All bacteria contain a protein called YidC that inserts proteins into the plasma membrane of bacterial cells. At present, a mechanistic understanding of the function of YidC, as well as its mitochondrial and chloroplast counterparts Oxa1 and Alb3, respectively, is limited by a lack of structural information. Furthermore, the region(s) of YidC mediating the interaction with the ribosome have not been identified, and the oligomeric state of YidC during co-translational translocation remains controversial. In the resulting model, the conserved membrane integrated core of YidC forms a helical bundle arranged like the vertices of a pentagon, in the order 4-5-3-2-6 (clockwise) when viewed from the cytoplasm.

In order to provide a molecular model of YidC in its active state, we reconstituted purified full length YidC (extended with the C-terminus of R. baltica YidC [Seitl et al., 2014]) with ribosome nascent chains (RNCs) exposing the first TM helix of FOc, and subjected the complex to cryo-EM and single particle analysis to a resolution of ∼8 Å. In agreement with previous structural studies, YidC binds to the ribosomal exit site, however, the improved resolution now allows for a more detailed interpretation. Secondly, the presence of elongated structural features allowed us to dock our molecular model in a distinct orientation (cross correlation coefficient 0.865). Following placement of the YidC-core model, two prominent densities in the membrane region, one next to TM3 and one next to TM5, remained unaccounted for. Given that (i) YidC substrates are known to crosslink to TM3, and (ii) that the density neighboring TM3 is aligned with the ribosomal exit tunnel and (iii) that at the same relative position nascent chains have been observed inside the SecY channel, the most plausible assignment to the density near TM3 appeared to be the TM helix of FOc. To verify this, and to exclude that the density neighboring TM5 corresponds to the nascent chain, we reconstituted single cysteine mutants of YidC either in TM3 (M430C and P431C) or in TM5 (V500C and T503C) with RNCs of a single cysteine mutant of FOc(G23C), and exposed them to disulphide crosslinking. Thus, the adduct represented indeed the inserting FOc TM domain crosslinked to TM3 of YidC. Indeed, mutation of residues Y370A and Y377A (contacting ribosomal RNA helix 59) and D488K (contacting ribosomal protein uL23) severely interfere with YidC activity thereby emphasizing their functional significance. Finally, it is notable that we observe only a single monomer of YidC bound to the active ribosome. While SecY is known to translocate hydrophilic nascent chains through its central aqueous channel and insert TM domains through a lateral gate, our model suggests that the YidC substrates are inserted at the protein-lipid interface.

> MDSQRNLLVIALLFVSFMIWQAWEQDKNPQPQAQQTTQTTTTAAGSAADQGVPASGQGKLISVKTDVLDLTINTRGGDVEQALLPAYPKELNSTQPFQLLETSPQFIYQAQSGLTGRDGPDNPANGPRPLYNVEKDAYVLAEGQNELQVPMTYTDAAGNTFTKTFVLKRGDYAVNVNYNVQNAGEKPLEISSFGQLKQSITLPPHLDTGSSNFALHTFRGAAYSTPDEKYEKYKFDTIADNENLNISSKGGWVAMLQQYFATAWIPHNDGTNNFYTANLGNGIAAIGYKSQPVLVQPGQTGAMNSTLWVGPEIQDKMAAVAPHLDLTVDYGWLWFISQPLFKLLKWIHSFVGNWGFSIIIITFIVRGIMYPLTKAQYTSMAKMRMLQPKIQAMRERLGDDKQRISQEMMALYKAEKVNPLGGCFPLLIQMPIFLALYYMLMGSVELRQAPFALWIHDLSAQDPYYILPILMGVTMFFIQKMSPTTVTDPMQQKIMTFMPVIFTVFFLWFPSGLVLYYIVSNLVTIIQQQLIYRGLEKRGLHSREKKKS;> MENLNMDLLYMAAAVMMGLAAIGAAIGIGILGGKFLEGAARQPDLIPLLRTQFFIVMGLVDAIPMIAVGLGLYVMFAVA> GPLGSPYTIELIQPEDGEAVIAMLKTFF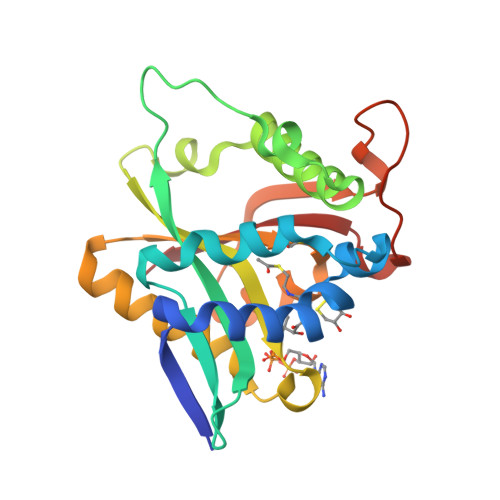FKDDPLNTFLDLGECKELEKYSLKPLPDNCSYKAVNKKGEIIGVFLNGLMRRPSPDDVPEKAADSCEHPKFKKILSLMDHVEEQFNIFDVYPDEELILDGKILSVDTNYRGLGIAGRLTERAYEYMRENGINVYHVLCSSHYSARVMEKLGFHEVFRMQFADYKPQGEVVFKPAAPHVGIQVMAKEV3-[methyl-[2-[methyl-(1-methylpiperidin-4-yl)amino]thieno[3,2-d]pyrimidin-4-yl]amino]propanenitrile | C17 H24 N6 S | 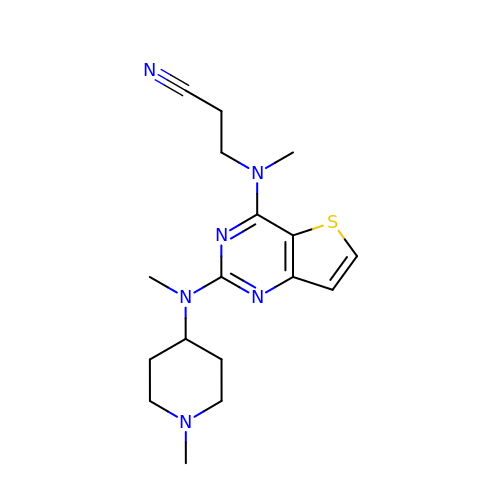JVWILFYYJUGFPA-UHFFFAOYSA-N>MAKIIGGFAVSHTPTIAFAHDANKYDDPVWAPIFQGFEPVKQWLAEQKPDVTFYVYNDHMTSFFEHYSHFALGVGEEYSPADEGGGQRDLPPIKGDPELAKHIAECLVADEFDLAYWQGMGLDHGAFSPLSVLLPHEHGWPCRIVPLQCGVLQHPIPKARRFWNFGRSLRRAIQSYPRDIKVAIAGTGGLSHQVHGERAGFNNTEWDMEFMERLANDPESLLGATVTDLAKKGGWEGAEVVMWLLMRGALSPEVKTLHQSYFLPSMTAIATMLFEDQGDAAPPAESDEALRARAKRELAGVEEIEGTYPFTIDRAVKGFRINHFLHRLIEPDFRKRFVEDPEGLFAESDLTEEEKSLIRNRDWIGMIHYGVIFFMLEKMAAVLGIGNIDVYAAFRGLSVPEFQKTRNAAITYSVAGKQ[2x]

The three catecholic compounds are degraded by three evolutionarily related type II extradiol dioxygenases–DesB, LigAB, and DesZ–in S. sp. SYK-6. On the other hand, DesB exhibits not only a strict substrate specificity but also high enzyme activity for gallate. While LigAB is an α2β2-type tetramer, DesB is a β2-type homo-dimer. In this study, we analyzed the mechanism of the substrate recognition of DesB on the basis of the crystal structures of reaction intermediates.

Interestingly, a large shift of the Fe (II) ion was observed in the DesB-gallate complex. The shift of the Fe (II) ion, which seems to be critical to the catalytic reaction, is likely to be induced by the substrate binding at the productive binding site and to cause the strict substrate specificity of DesB. On the other hand, the Fe (II) ion at the A-site is located at a distance of approximately 2 Å from the R-site and coordinates OH and OH of gallate. The crystallographic analysis in this study showed alternative conformations of the Fe (II) ion, R- and A-sites, both in C2221 and P21 crystals. Interestingly, no crystal structures showed 100% occupancy of the Fe (II) ion at the A-site. The observation of the alternative conformation of the Fe (II) ion could be explained by a hypothesis that the shift of the Fe (II) ion is reversible under anaerobic conditions. Analysis of the van der Waals surface around the active site showed that direct coordination between the hydroxyl groups of gallate and the Fe (II) ion at the R-site cannot be allowed due to steric hindrance. For the direct coordination, the Fe (II) ion should be shifted as observed in the DesB-gallate complex. We therefore concluded that the shift of the Fe (II) ion from the R- to A-sites is required for direct coordination between the Fe (II) ion and the substrate. In addition, the catalytic reaction of DesB requires the shift of the Fe (II) ion, leading to the bidentate coordination of the substrate to the Fe (II) ion.>[3x]GCGCGGCGAUUUAACCGUAUUGCAG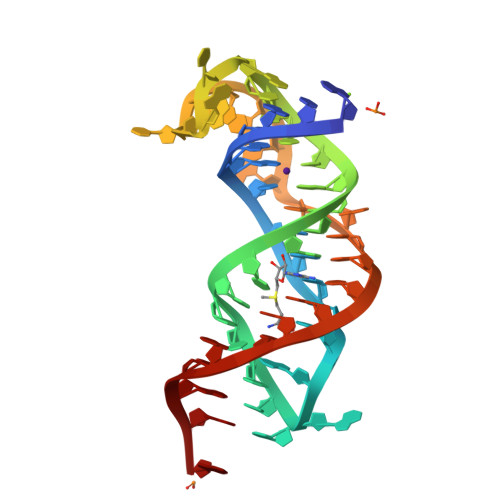UCGCGUGAUAAAUGUAGCUAAAAAGGA> GHMGPATKDIPDVAGQTVDV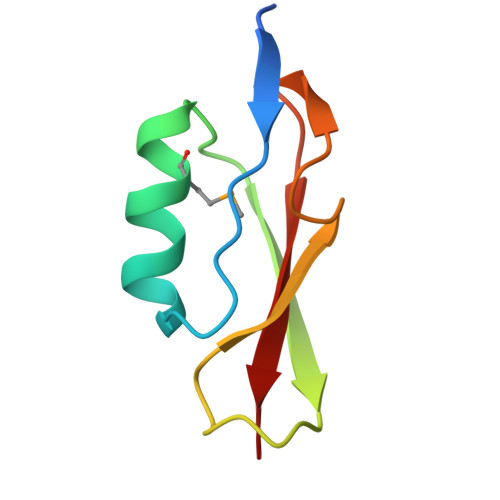AQKNMNVYGFTKFSQASVDSPRPAGEVTGTNPPAGTTVPVDSVIELQVSKG> GPDSMAMEMRLPVAR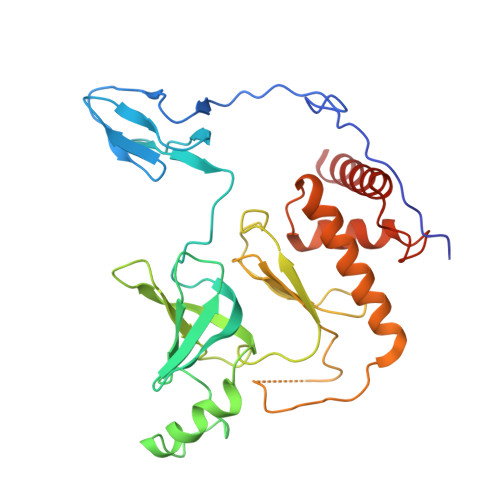KPLSERLGRDTKKHLVVPGDTITTDTGFMRGHGTYMGEEKLIASVAGSVERVNKLICVKALKTRYIGEVGDIVVGRITEVQQKRWKVETNSRLDSVLLLSSMNLPGGELRRRSAEDELAMRGFLQEGDLISAEVQAVFSDGAVSLHTRSLKYGKLGQGVLVQVSPSLVKRQKTHFHDLPCGASVILGNNGFIWIYPTPEHKEEEAGGFIANLEPVSLADREVISRLRNCIISLVTQRMMLYDTSILYCYEASLPHQIKDILKPEIMEEIVMETRQRLLEQEG> MNV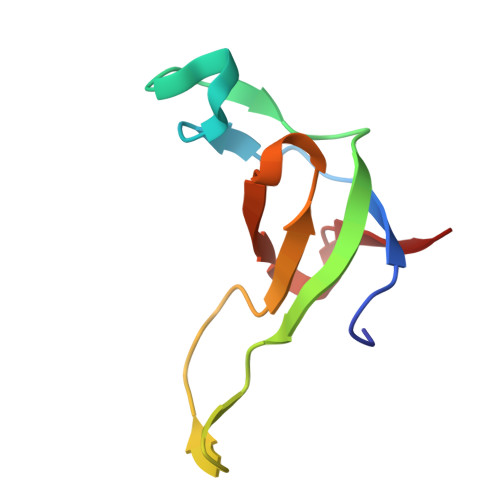GDRVRVTSSVVVYHHPEHKKTAFDLQGMEGEVAAVLTEWQGRPISANLPVLVKFEQRFKAHFRPDEVTLI> MSKFLDRFRYFKQKGETFADGHGQLLNTNRDWEDGYRQRWQHDKIVRSTHGVNCTGSCSWKIYVKNGLVTWETQQTDYPRTRPDLPNHEPRGCPRGASYSWYLYSANRLKYPMMRKRLMKMWREAKALHSDPVEAWASIIEDADKAKSFKQARGRGGFVRSSWQEVNELIAASNVYTIKNYGPDRVAGFSPIPAMSMVSYASGARYLSLIGGTCLSFYDWYCDLPPASPQTWGEQTDVPESADWYNSSYIIAWGSNVPQTRTPDAHFFTEVRYKGTKTVAVTPDYAEIAKLCDLWLAPKQGTDAAMALAMGHVMLREFHLDNPSQYFTDYVRRYTDMPMLVMLEERDGYYAAGRMLRAADLVDALGQENNPEWKTVAFNTNGEMVAPNGSIGFRWGEKGKWNLEQRDGKTGEETELQLSLLGSQDEIAEVGFPYFGGDGTEHFNKVELENVLLHKLPVKRLQLADGSTALVTTVYDLTLANYGLERGLNDVNCATSYDDVKAYTPAWAEQITGVSRSQIIRIAREFADNADKTHGRSMIIVGAGLNHWYHLDMNYRGLINMLIFCGCVGQSGGGWAHYVGQEKLRPQTGWQPLAFALDWQRPARHMNSTSYFYNHSSQWRYETVTAEELLSPMADKSRYTGHLIDFNVRAERMGWLPSAPQLGTNPLTIAGEAEKAGMNPVDYTVKSLKEGSIRFAAEQPENGKNHPRNLFIWRSNLLGSSGKGHEFMLKYLLGTEHGIQGKDLGQQGGVKPEEVDWQDNGLEGKLDLVVTLDFRLSSTCLYSDIILPTATWYEKDDMNTSDMHPFIHPLSAAVDPAWEAKSDWEIYKAIAKKFSEVCVGHLGKETDIVTLPIQHDSAAELAQPLDVKDWKKGECDLIPGKTAPHIMVVERDYPATYERFTSIGPLMEKIGNGGKGIAWNTQSEMDLLRKLNYTKAEGPAKGQPMLNTAIDAAEMILTLAPETNGQVAVKAWAALSEFTGRDHTHLALNKEDEKIRFRDIQAQPRKIISSPTWSGLEDEHVSYNAGYTNVHELIPWRTLSGRQQLYQDHQWMRDFGESLLVYRPPIDTRSVKEVIGQKSNGNQEKALNFLTPHQKWGIHSTYSDNLLMLTLGRGGPVVWLSEADAKDLGIADNDWIEVFNSNGALTARAVVSQRVPAGMTMMYHAQERIVNLPGSEITQQRGGIHNSVTRITPKPTHMIGGYAHLAYGFNYYGTVGSNRDEFVVVRKMKNIDWLDGEGNDQVQESVK;> MKIRSQVGMVLNLDKCIGCHTCSVTCKNVWTSREGVEYAWFNNVETKPGQGFPTDWENQEKYKGGWIRKINGKLQPRMGNRAMLLGKIFANPHLPGIDDYYE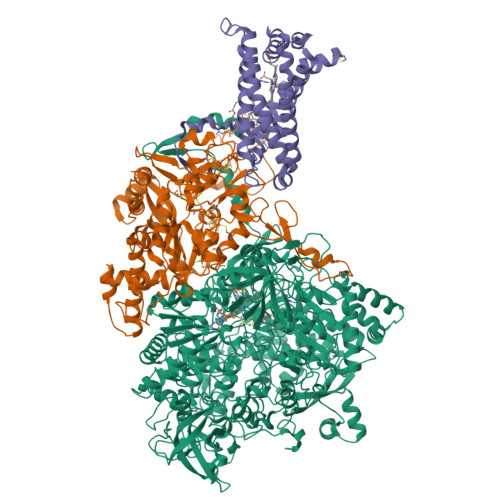PFDFDYQNLHTAPEGSKSQPIARPRSLITGERMAKIEKGPNWEDDLGGEFDKLAKDKNFDNIQKAMYSQFENTFMMYLPRLCEHCLNPACVATCPSGAIYKREEDGIVLIDQDKCRGWRMCITGCPYKKIYFNWKSGKSEKCIFCYPRIEAGQPTVCSETCVGRIRYLGVLLYDADAIERAASTENEKDLYQRQLDVFLDPNDPKVIEQAIKDGIPLSVIEAAQQSPVYKMAMEWKLALPLHPEYRTLPMVWYVPPLSPIQSAADAGELGSNGILPDVESLRIPVQYLANLLTAGDTKPVLRALKRMLAMRHYKRAETVDGKVDTRALEEVGLTEAQAQEMYRYLAIANYEDRFVVPSSHRELAREAFPEKNGCGFTFGDGCHGSDTKFNLFNSRRIDAIDVTSKTEPHP;> MQFLNMFFFDIYPYIAGAVFLIGSWLRYDYGQYTWRAASSQMLDRKGMNLASNLFHIGILGIFVGHFFGMLTPHWMYEAWLPIEVKQKMAMFAGGASGVLCLIGGVLLLKRRLFSPRVRATTTGADILILSLLVIQCALGLLTIPFSAQHMDGSEMMKLVGWAQSVVTFHGGASQHLDGVAFIFRLHLVLGMTLFLLFPFSRLIHIWSVPVEYLTRKYQLVRARH>KETAAAKFERQHMDSGNSPSSSSNYCNQMMCCRNLTKDRCKPVNTFVHESLADVQAVCSQKNVACKNGQTNCYQSYSTMSITDCRETGSSKYPNCAYKTT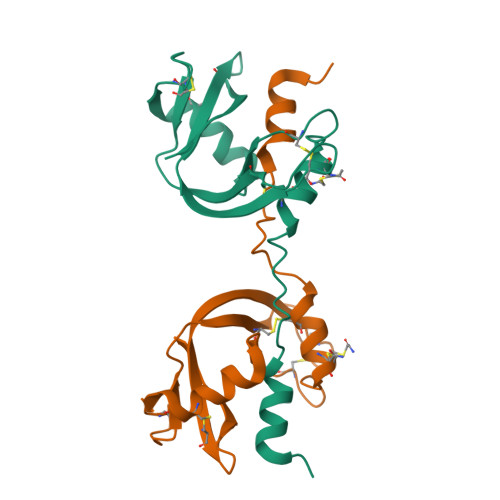QANKHIIVACEGNPYVPVHFDASV[2x]>[4x]MRKFDKSIAAFEEAQDLMPGGVNSPVRAFKSVGMNPLFMERGKGSKVYDIDGNEYIDYVLSWGPLIHGHANDRVVEALKAVAERGTSFGAPTEIENKLAKLVIERVPSIEIVRMVNSGTEATMSALRLARGYTGRNKIL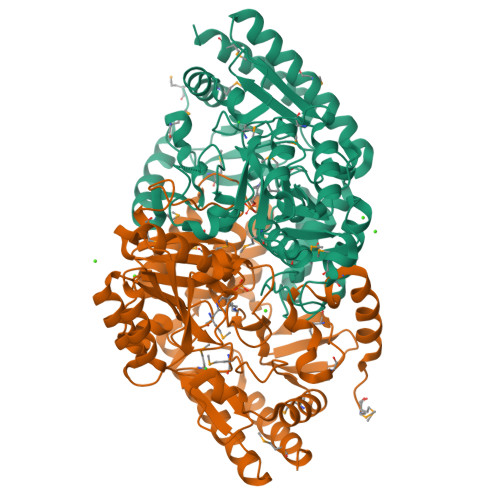KFIGCYHGHGDSLLIKAGSGVATLGLPDSPGVPEGVAKNTITVAYNDLESVKYAFEQFGDDIACVIVEPVAGNMGVVPPQPGFLEGLREVTEQNGALLIFDEVMTGFRVAYNCGQGYYGVTPDLTCLGKVIGGGLPVGAYGGKAEIMRQVAPSGPIYQAGTLSGNPLAMAAGYETLVQLTPESYVEFERKAEMLEAGLRKAAEKHGIPHHINRAGSMIGIFFTDEPVINYDAAKSSNLQFFAAYYREMVEQGVFLPPSQFEGLFLSTVHSDADIEATIAAAEIAMSKLKA>[4x]LVPRGSHMLESYAFNMKATVEDEKLQG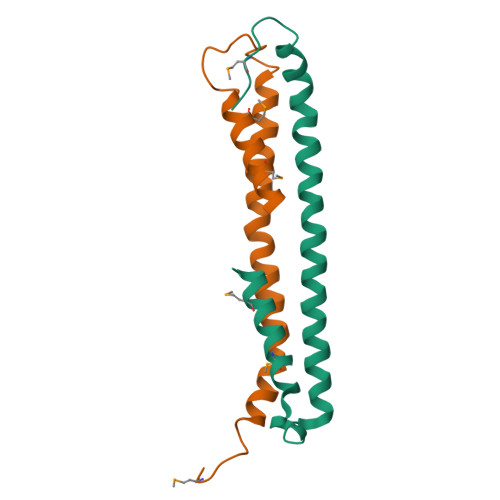KINDEDKQKILDKCNEIISWLDKNQTAEKEEFEHQQKELEKVCNPIITKLYQSAGGMPGGMPGGFPGGGAPPSGGASSGPTIEEVD3-[(4-AMINO-1-TERT-BUTYL-1H-PYRAZOLO[3,4-D]PYRIMIDIN-3-YL)METHYL]PHENOL 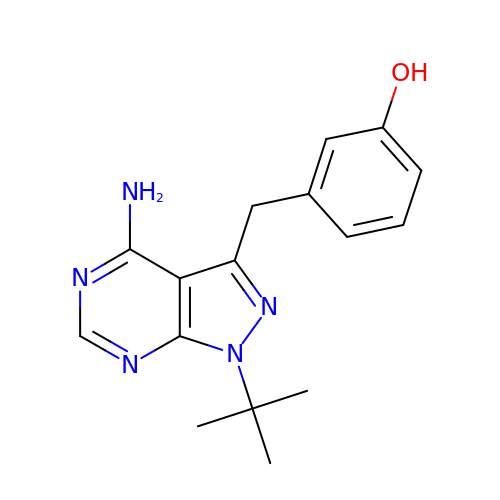| C16 H19 N5 O | QMAIQPBRCNEJAT-UHFFFAOYSA-N> LSISAVQRRYRLFHPVHQTVPFHFNPVQSIFPLIYENNLLAKPRLSWKDYEGRKEFDADHPLPVVGTR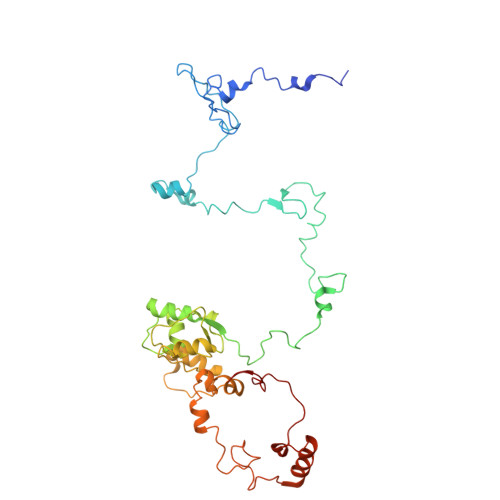LNERTTTHKWSHWDQYINPQITQSWMYLTQTPEYVGPRSGHNVIKMGWMKIGGSWKYSRSYNDARRGFAKGQWQERKMTPRFMLAPRVSAGGPRNRYEGKASFSRLSLSKLLWAVDTGRLNPNETITLYHLRNAKVIADREVVWPGMVLLAGNVERVPYPLHIELQNASAKAIQLLEEAGGSFTNVYMSHEGLYQELHPEEFPTFMEQELPERKGLENFATNSRKRGWLAQWYEDESRYAHPGAGRRTAHYIRPPTDRDFPATIEEYELAKHHQKWHLNQPGSATVLPWHSLNTADMARRSAGRL>[2x]GSNRTLIVTTILEEPYVMYRKSDKPLYGNDRFEGYCLDLLKELSNILGFLYDVKLVPDGKYGAQNDKGEWNGMVKELIDHRADLAVAPLTITYVREKVIDFSKP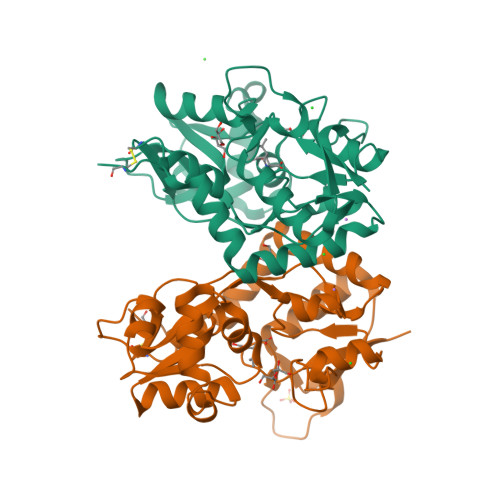FMTLGISILYRKGTPIDSADDLAKQTKIEYGAVRDGSTMTFFKKSKISTYEKMWAFMSSRQQSALVKNSDEGIQRVLTTDYALLMESTSIEYVTQRNCNLTQIGGLIDSKGYGVGTPIGSPYRDKITIAILQLQEEGKLHMMKEKWWRGNGCPE>GSAVVALTNDRDTSYFGEIGIGTPPQKFTVIFDTGSSVLWVPSSKCINSKACRAHSMYESSDSSTYKENGTFGAIIYGTGSITGFFSQDSVTIGDLVVKEQDFIEATDEADNVFLHRLFDGILGLSFQTISVPVWYNMLNQGLVKERRFSFWLNRNVDEEEGGELVFGGLDPNHFRGDHTYVPVTYQYYWQFGIGDVLIGDKSTGFCAPGCQAFADSGTSLLSGPTAIVTQINHAIGAN[2x];>EELQVDCNTLSSMPNVSFTIGGKKFGLTPEQYILKVGKGEATQCISGFTAM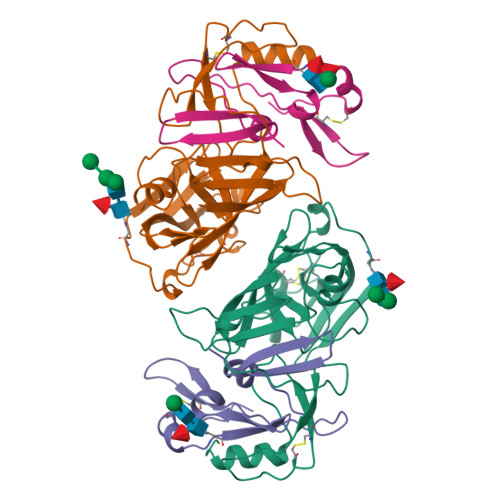DATLLGPLWILGDVFMRPYHTVFDYGNLLVGFAEAA[2x]> GFPTELKPGTNQFLTTDDGVSAPILPNFHPTPCIHIPGEVRNLLELCQVETILEVNNVPTNATSLMERLRFPVSAQAGKGELCAVFRADPGRSGPWQSTLLGQLCGYYTQWSGSLEVTFMFTGSFMATGKMLIAYTPPGGPLPKDRATAMLGTHVIWDFGLQSSVTLVIPWISNTHYRAHARDGVFDYYTTGLVSIWYQTNYVVPIGAPNTAYIIALA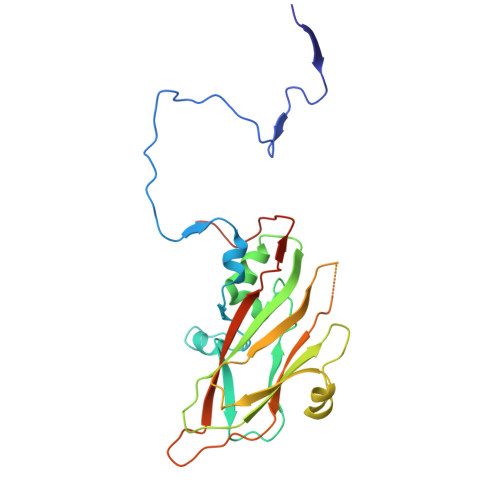AAQKNFTMQLCKDASDILQTGTIQ>[60x]AGGVGVSTGDFDNTTLWDFHEDGTATITCNSTRLVHLTRPDSLDY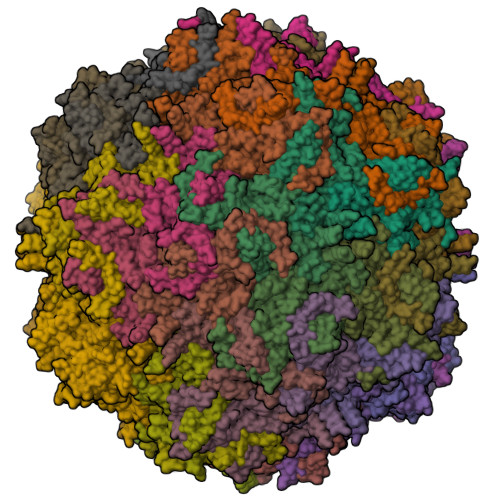KIIPTQNNTAVQTVGHMMDDDNHTQVLTPWSLVDCNAWGVWLSPHDWQHIMNIGEELELLSLEQEVFNVTLKTATETGPPESRITMYNNDLTAVMMITTDTNNQLPYTPAAIRSETLGFYPWRPTVVPRWRYYFDWDRFLSVTSSSDQSTSIINHSSTQSAIGQFFVIETQLPIALLRTGDSYATGGYKFDCNKVNLGRHWQTTRSLGLPPKIEPPTSESALGTINQNARLAWRWGINDVHETNVVRPCTAGYNHPEWFYTHTLEGPAIDPAPPTSIPSNWGGGTPPDTRASSHNQQRITYNYNHGNKDENLNNFSLNPNNIEGSIINQGNFLSYEGNGQQINTTAGVAKNGETATSDPNLVRYMPNTYGVYTAVDHQGPVYPHGQIWDKQIHTDKKPELHCLAPFTCKNNPPGQMFVRIAPNLTDTFNATPTFSEIITYADFWWKGTLKMKIKLRPPHQWNIATVLGAAVNIGDAARFVPNRLGQLEFPVINGRIVPSTVY> NRRRTWTNRPMYRKPRLYRMYRTPDVPKGCEGPCKVQSYEQRHDISHVG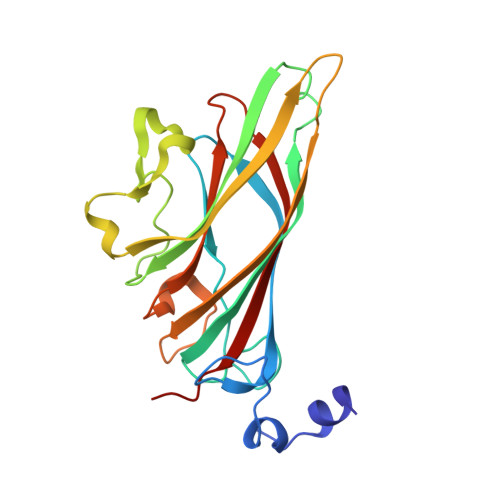KVLCVSDVTRGNGLTHRVGKRFCVKSVYVLGKIWMDENIKTKNHTNTVMFYLVRDRRPFGTAMDFGQVFNMYDNEPSTATIKNDLRDRYQVLRKFTSTVTGGQYASKEQALVKKFMKINNYVVYNHQEAAKYDNHTENALLLYMACTHASNPVYATLKIRIYFYDSVQN> RPWSEFRLTPAEAAAAAALAARCAQRYDETDGPEFLLDAPVIAHELPRRLRTFMARARLDAWPHALVVRGNPVDDAALGSTPVHWRTARTPGSRPLSFLLMLYAGLLGDVFGW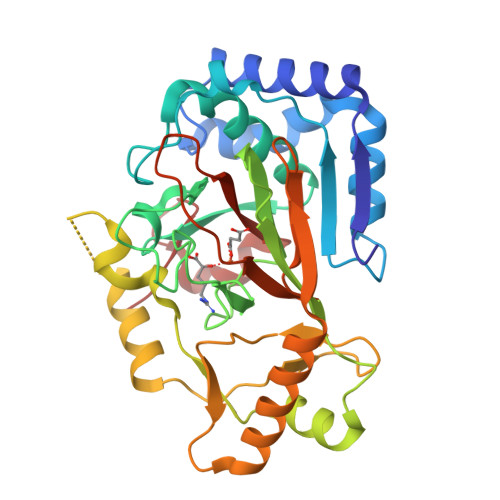ATQQDGRVVTDVLPIKGGEHTLVSSSSRQELGWHTEDAFSPYRADYVGLLSLRNPDGVATTLAGVPLDDLDERTLDVLFQERFLIRPDDSHLQVNNSTAQQGRVEFEGIAQAADRPEPVAILTGHRAAPHLRVDGDFSAPAEGDEEAAAALGTLRKLIDASLYELVLDQGDVAFIDNRRAVHGRRAFQPRYDGRDRWLKRINITRDLHRSRKAWAGDSRVLGQR>[2x]AEEWYFGKITRRESERLLLNPE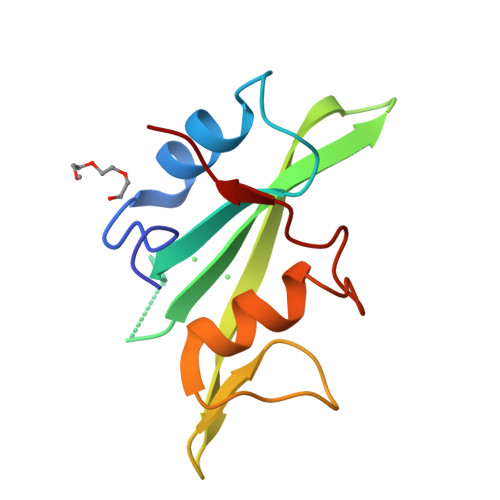NPRGTFLVRESETTKGAYCLSVSDFDNAKGLNVKHYKIRKLDSGGFYITSRTQFSSLQQLVAYYSKHADGLCHRLTNVCPT;> PQYIYVPA>[3x]MAHHHHHHMATIRIQTDDFDLNAEVAALRARNPKIGALACFVGTV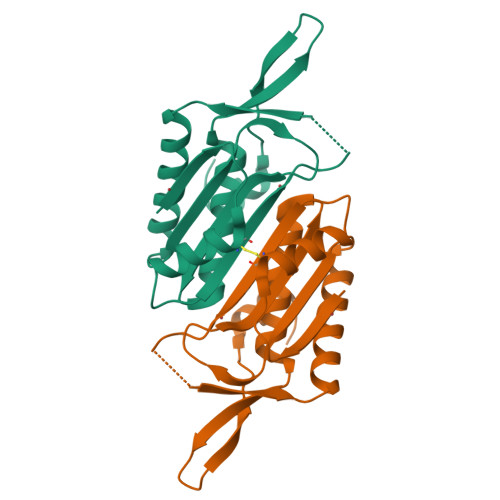RDLNEGDSVAAMELEHYPGMTEKALEKIAAEAGRRWPGIDVAIVHRVGRLLPLDQIVMVATVASHRGDAFASCEFVMDYLKTEAPFWKKETTPDGERWVDARSTDDAALARWGVESGNTPR> MLEQMISSSKVGVKINEWYKYIRLFSVPDSEILKAEVEEEIRHMKEDHDLLLYYSLMCFRHQLMLDYLEPK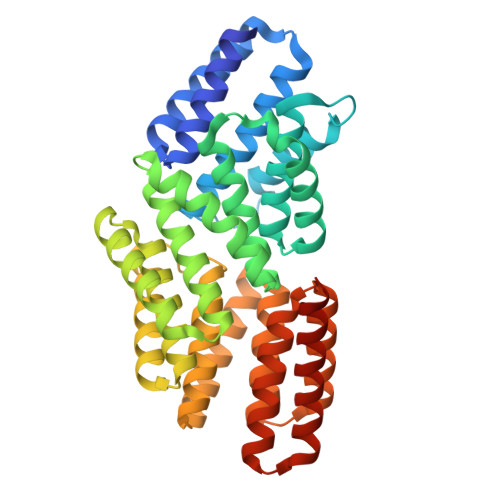TLNEERPKISDLLEKIESSQTDLKGILEYYFNFFRGMYEFEQYEYLNAISFYKQAERKLSLVADEIERAEFHYKVAEIYYHMKQTHMSMHHIVQAIDSYKAHENYTVRVIQCSFVIGLNYLDMDYPEKAIPHFKNALDKAREIDMSRLIGSSLYNLGLCSFAEEAYEKASEYFKEGIRVYQDNGYEHSNRILDILLMLTKTTFKMRNHSEGISWCAHGLSLSKNLNDEIMAKMFEFIHALYVDNDNEKLNSILNYLELKSMLSDVEDLASDAAKYYNEKEDHKVAVAYYEKVLYARKQIQRGDCLYET>[2x]AQGSHYKQIIKNDENITVNESVPRGRILDRNGKVLVDNASKMAITYTRGRKTTQSEMLDTAEKLSKLIKMDTKKITERDKKDFWIQLHPKKAKAMMTKEQAMLADGSIKQDQYDKQLLSKIRKSQLDELSSKDLQVLAIFREMNAGTVLDPQMIKNEDVSEKEYAAVSQQLSKLPGVNTSMDWDRKYPYGDTLRGIFGDVSTPAEGIPKELTEHYLSKGYSRNDRVGKSYLEYQYEDVLRGKKKEMKYTTDKSGKVTSSEVLNPGARGQDLKLTIDI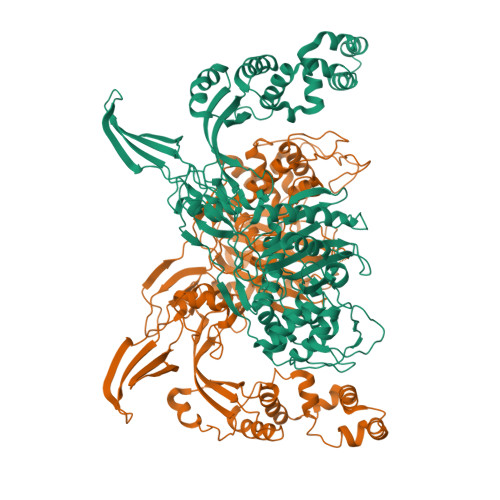DLQKEVEALLDKQIKKLRSQGAKDMDNAMMVVQNPKNGDILALAGKQINKSGKMTDYDIGTFTSQFAVGSSVKGGTLLAGYQNKAIKVGETMVDEPLHFQGGLTKRSYFNKNGHVSINDKQALMHSSNVYMFKTALKLAGDPYYSGMALPSDISSPAQKLRRGLNQVGLGVKTGIDLPNETRGQIEPLTNNPGNYLDLSIGQYDTYTPLQLSQYVSTIANDGYRIQPHIGLTIHESTNKDEVGPLKKKINGTVLNKVNNTEKEIKQIQEGFKMAFNDKDGTGYVSFKDTVVPTAGKTGTAEVFQNGEPRVNSTYIGYAPIDDPKLAFSIVYTNQPVPPPWLTGGDLGRDVINYYFKQLGKDDKNKDKDK>PKHGKRYRALLEKVDPNKIYTIDEAAHLVKELATAKFDETVEVHAKLGIDPRRSDQNVRGTVSLPHGGRIEFRNDKTGAIHAPVGKASFPPEKLADNIRAFIRALEAHKPEGAKGTFLRSVYVTTTMGPSV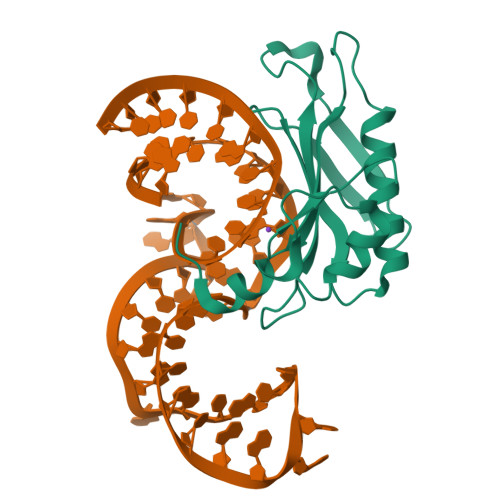RINPHS[2x]> STRDYEIQRERIELGRCIGEGQFGDVHQGIYMSPENPALAVAIKTCKNCTSDSVREKFLQEALTMRQFDHPHIVKLIGVITENPVWIIMELCTLGELRSFLQVRKYSLDLASLILYAYQLSTALAYLESKRFVHRDIAARNVLVSSNDCVKLGDFGLSRYMEDSTYYKASKGKLPIKWMAPESINFRRFTSASDVWMFGVCMWEILMHGVKPFQGVKNNDVIGRIENGERLPMPPNCPPTLYSLMTKCWAYDPSRRPRFTELKAQLSTILEEEKLQ

Focal Adhesion Kinase (FAK) is a non-receptor tyrosine kinase that regulates signals involved in cell proliferation, migration and survival. FAK activation is initiated by breaking an intramolecular autoinhibitory interaction between the N-terminal FERM (4.1, ezrin, radixin, moesin homology) and kinase domains. All compounds exhibit a common 5-chloro-2-ortho-methoxyanilino-4-anilinopyrimidine core structure, which binds in a nearly identical manner to the hinge region of the FAK kinase.

The structures reveal that the carbonyl in the carbamoyl moiety of TAE226 and an analogous carbonyl in 2 of the 3 other compounds stabilize an unusual helical conformation of the DFG motif. The carbonyl within the isoindoline moieties of TAF089 and TAF672 superimpose well with the carbonyl in TAE226 and induce a similar helical turn at the DFG motif. The morpholine (TAE226), methylpiperazine (TAF089), dipiperidine (TAF672) or methylaminopyrrolidine (AZW592) moieties in para position to the amine groups of the aniline rings make almost no protein contacts, consistent with their incorporation for improved pharmacokinetic properties of the respective compounds. IC50 values for TAF672 could not be reliably determined because of its low solubility in DMSO and aqueous buffers, however, it can be expected to mirror the potency of TAF089 since the moiety that interacts with the FAK kinase is identical for both inhibitors.>[2x]DAGDKGIYRHYMQKEIYEQPNAIKNTLTGRISHGQVDLSELGPNADELLSKVEH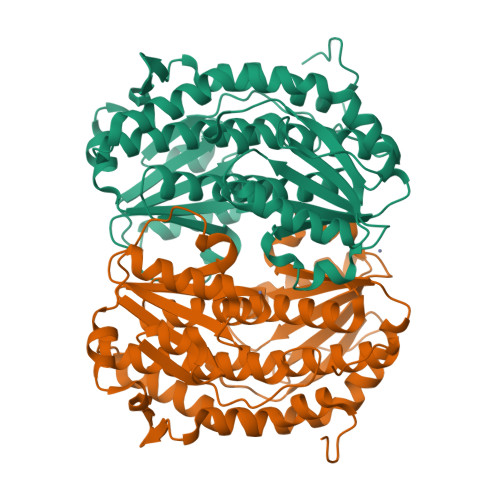IQILACGTSYNSGMVSRYWFESLAGIPCDVEIASEFRYRKSAVRRNSLMITLSQSGETADTLAGLRLSKELGYLGSLAICNVPGSSLVRESDLALMTNAGTEIGVASTKAFTTQLTVLLMLVAKLSRLKGLDASIEHDIVHGLQALPSRIEQMLSQDKRIEALAEDFSDKHHALFLGRGDQYPIALEGALKLKEISYIHAEAYAAGELKHGPLALIDADMPVIVVAPNNELLEKLKSNIEEVRARGGQLYVFADQDAGFVSSDNMHIIEMPHVEEVIAPIFYTVPLQLLAYHVALIKGTDVDQPRNLAKSVTVE1-beta-D-glucopyranosyl-4-(hydroxymethyl)-1H-1,2,3-triazole 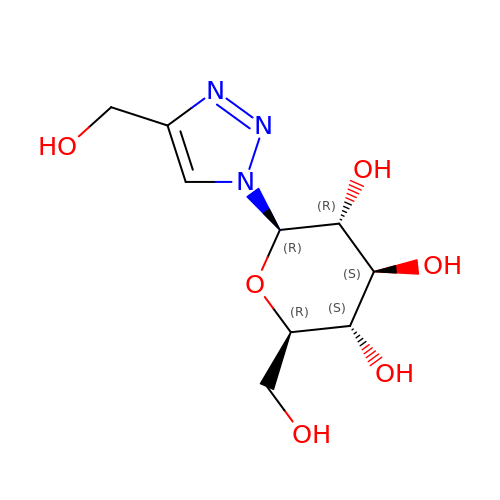| C9 H15 N3 O6 | BHGZOVXPACYZLI-SYHAXYEDSA-N>[2x]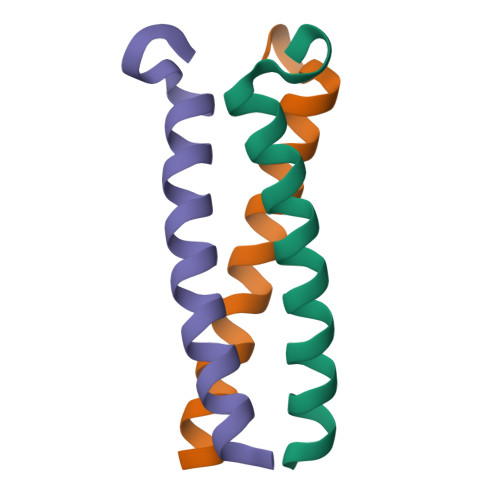XEVEALEKKVEALELKVQKLEKKVEALEHGWDGR VT-464 | C18 H17 F4 N3 O3 | 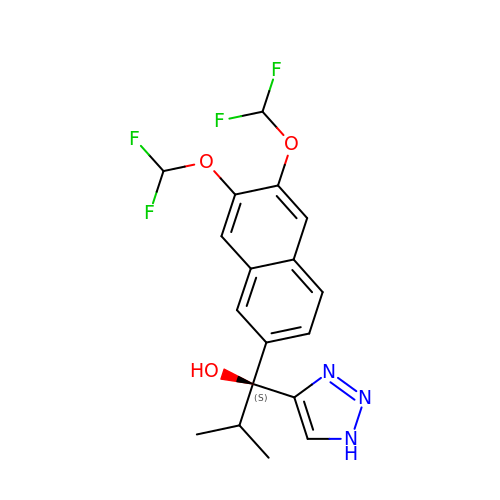ZBRAJOQFSNYJMF-SFHVURJKSA-N>[2x]MSYPAFDSKTFLEAHIEKTMAFYFPTCIDPEGGFFQFFKDDGSVYDPNTRHLVSSTRFIFNFAQAYLHTNIAEYKHAAVHGIQYLRQRHQSQSGGYVWLLDGGTNLDETNHCYGLAFVILAYSNALQIGLSEAEVWIEVTYDLL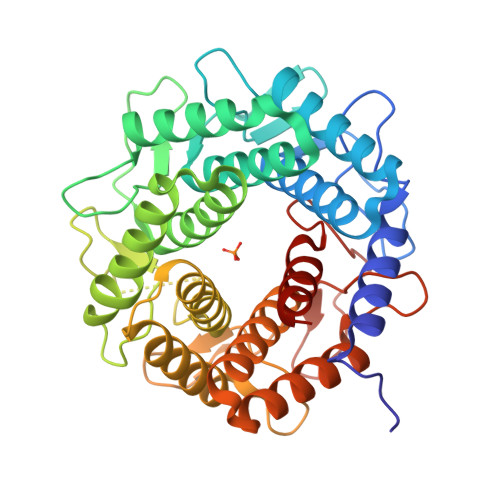ETHFWENKHGLYLDEISSDWKTVSPYRGQNANMHMCEALMSAFDATQNPKYLDRAKLLAKNICQKQASLSNSNEVWEHYTNDWQIDWDYNKNDPKHLFRPWGFQPGHQTEWAKLLLMLDKRSPENWYLPKAKYLFDLAYKKAWDTKKGGLHYGYAPDGTVCDPDKYFWVQAESFAAAWLLYKATKDETYYKQYLTLWEFSWNHMIDHTFGAWYRILDENNAQYDNNKSPAGKTDYHTMGACYEVLKTLTL>MTKNPRNNKPKKILDSSYKSKTIWQNYIDALFETFPQLEISEVWAKWDGGNVTKDGGDAKLTANIRTGEHFLKAREAHIVDPNSDIYNTILYPKTGADLPCFGMDLMKFSDKKVIIVFDFQHPREKYLFSVDGLPEDDGKYRFFEM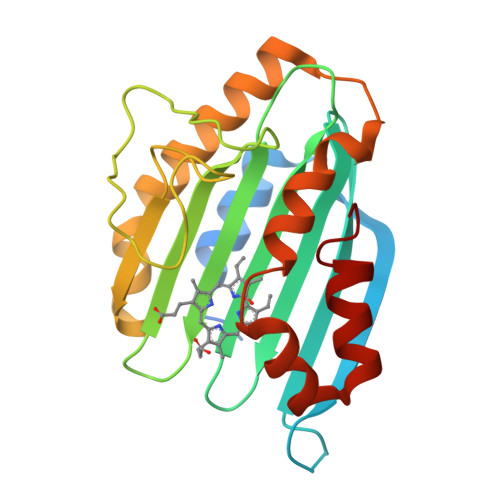GNHFSKNIFVRYCKPDEVDQYLDTFKLYLTKYKEMIDNNKPVGEDTTVYSDFDTYMTELDPVRGYMKNKFGEGRSEAFVNDFLFSYK[4x]>MAHHHHHHVGTDDWRCARSMHEFSLKDIDGHMVNLDKYRGFVVILTNVASQCGKTEVNYTQLVDLHARYAECGLRILAVPCNQFGKQEPGSNEEIKEFAAGYNVKFDMFSKACVNGDDAHPLFKWMKIQPKGKGI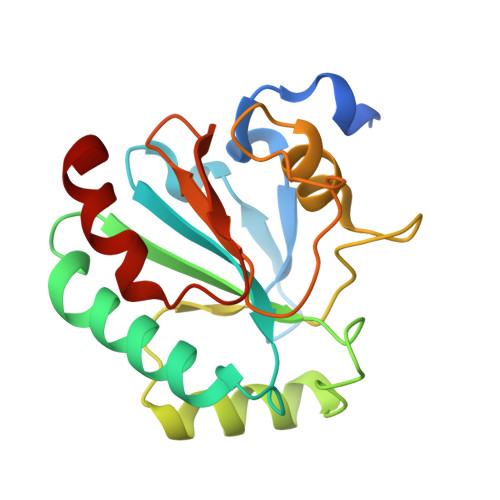LGNAIKWNFTKFLIDKNGCVVKRYGPMEEPLVIEKDLPHYF[4x]6-[2-[4-[2-(3,4-dichlorophenyl)ethyl]piperazin-1-yl]phenyl]-~{N}-(3-pyrrolidin-1-ylpropyl)-2~{H}-pyrazolo[3,4-b]pyridine-4-carboxamide 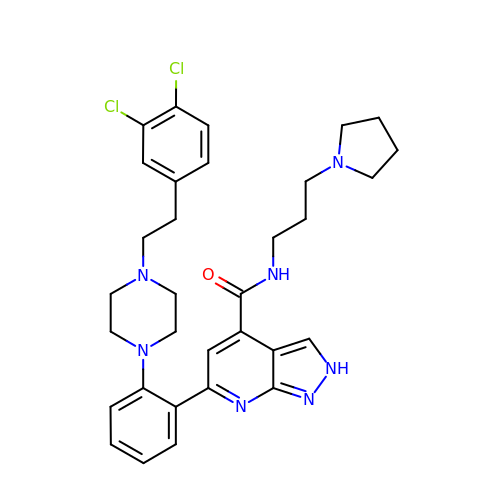| C32 H37 Cl2 N7 O | UYKVPOQVUKTFDL-UHFFFAOYSA-N>MSGFKFLFFSPDGTLYGVHNDKLYKGTPPTSDKDNWLARATLIGNGGW[10x]

We describe complex formation between a designed pentameric β-propeller and the anionic macrocycle sulfonato-calix[8]arene (sclx8), as characterized by X-ray crystallography and NMR spectroscopy. Each blade of this β-propeller is a 47-residue monomer of ∼5.2 kDa (yielding a pentamer of ∼26 kDa) that binds one equivalent of N-acetylglucosamine (GlcNAc). The Asn33Lys mutation makes the protein cationic, with a calculated isoelectric point, pI ∼ 8. As is typical of β-propellers, Pent has a toroidal structure with a funnel-like central channel.

Despite their unusual morphology, diffraction data extending to 1.6 Å resolution were collected from the crystals grown in the presence of MgCl2. This structure was solved in space group P1211 with an asymmetric unit comprising two Pent molecules and one sclx8. The calixarene, evident in the unbiased electron density map, is sandwiched between two molecules of Pent arranged as a dimer. This dimer assembles via the concave pockets of each protein, with the Ser2 and Asp21 side chains on each subunit contributing to the Pent–Pent interface. Although the concave pocket is the calixarene binding site, due to steric constraints, only one sclx8 can be accommodated within the Pent dimer. One of the protein–calixarene interfaces is similar to form I, while the “capping” protein has fewer interactions with the calixarene and an ∼2-fold smaller interface area. The calixarene was refined at 60% occupancy and with high B-factors (∼50 Å2 vs ∼30 Å2 for the protein), which may be due to fluxionality of the macrocycle between the two binding sites available in the Pent–Pent dimer. The increased ionic strength of the crystallization conditions in form II (including 50 mM MgCl2 or 0.1 M Bis-Tris) versus form I may have altered the protein–calixarene assembly in favor of protein dimerization. While sclx8 is a well-established host macrocycle in supramolecular chemistry, it behaves as a guest sitting in the host Pent. This hosting action of the protein is emphasized in crystal form II, where a Pent dimer encapsulates one sclx8.>[2x]GMSLDNDSLHLPKYDDFVQSISVLALTMSGSELHGIMCGYLCAGADSQGEAYIRALLNNKKDEQSRNALLSMFSVFSIS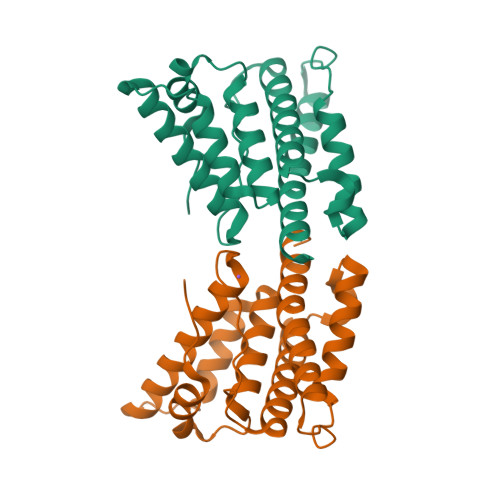QQQMNNFDFEFEMLLPDDDESLVTRAQAFSEWCEGFTQGLTIAGVGMEQFYEEESQDALQHLMEFAELDCESLEVGEEDERALMEVSEYTRMAVLRLHSDLVLHERELGDSGTTH>AYTTFSQTKNDQLKEPMFFGQPVNVARYDQQKYDIFEKLIEKQLSFFWRPEEVDVSRDRIDYQALPEHEKHIFISNLKYQTLLDSIQGRSPNVALLPLISIPELETWVETWAFSETIHSRSFTHIIRNIVNDPSVVFDDIVTNEQIQKRAEGISSYYDELIEMTSYWHLLGEGTHTVNGKTVTVSLRELKKKLYLCLMSVNALEAIRAYVSFACSFAFAERELMEGNAKIIRLIARDEALHLTGTQHMLNLLRSGADDPEMAEIAEECKQECYDLFVQAAQQEKDWADYLFRDGSMIGLNKDILCQYVEYITNIRMQAVGLDLPFQTRSNPIPWINTWLV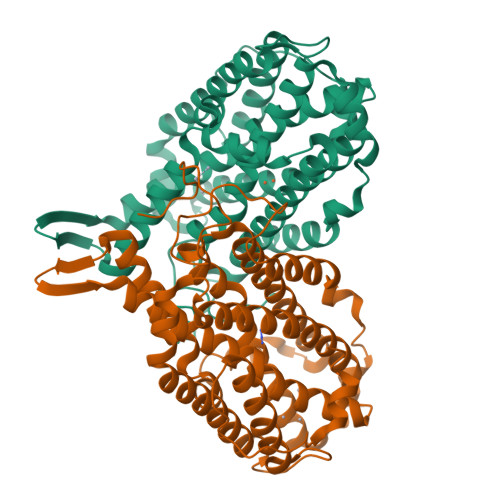SDNVQVAPQEVEVSSYLVGQIDSEVDTDDLSNFQL[2x]> GCCSHPACNV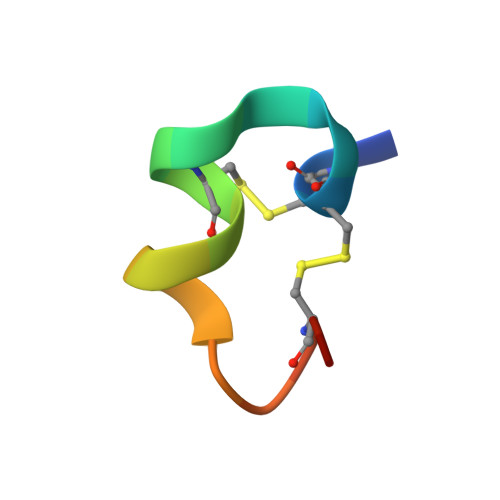NNPHICGX> MGEEAELAYLLGELAYKLGEYRIAIRAYRIALKRDPNNAEAWYNLGNAYYKQGDYDEAIEYY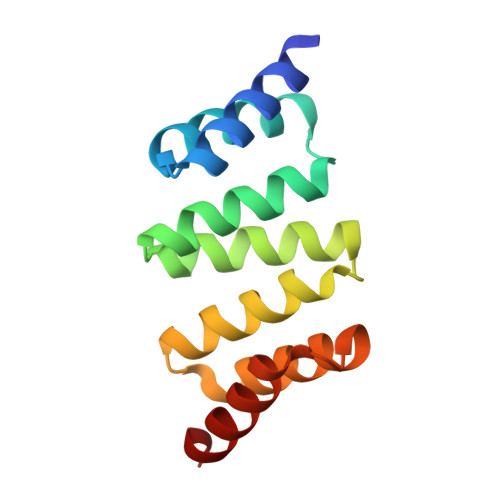QKALELDPNNAEAWYNLGNAYYKQGDYDEAIEYYEKALELDPENLEALQNLLNAMDKQG Here, we report the identification of NADases on the surface of fungi such as the pathogen Aspergillus fumigatus and the saprophyte Neurospora crassa. The enzymes harbour a tuberculosis necrotizing toxin (TNT) domain and are predominately present in pathogenic species. Interestingly, N. crassa NADase (NcNADase) activity was not affected by either EGTA or Ca2+. Both AfNADase and NcNADase cleaved NAD+ and NADP+, but not their reduced counterparts, NADH and NADPH. The absence of ADP-ribosyl cyclase activity from the fungal NADase was further substantiated by its inability to convert the NAD+ analogue nicotinamide hypoxanthine dinucleotide (NHD+) to Nam and fluorescent N7-cyclic inosine diphosphoribose (N7-cIDPR), a reaction specifically observed for cyclases. These results demonstrate that fungal NADases are pure NAD glycohydrolases as they lack both cyclase and base-exchange activity.

The 1.6 Å X-ray structure of the homodimeric A. fumigatus protein reveals unique properties including N-linked glycosylation and a Ca2+-binding site whose occupancy regulates activity. The protein crystallizes in the space group P3221 with two molecules in the asymmetric unit confirming the homodimeric assembly suggested from the chromatographic analysis. The dimeric assembly is formed via an interface of 2260 Å2 of the total solvent-accessible area of 11030 Å2 (calculated with PDBePISA server), involving 66 residues, including the C-terminus which is intertwined with the other protomer. The protomers consist of two domains, an N-terminal ‘thumb’ and a C-terminal ‘palm’ domain. The thumb domain, residues 20-117, is folded containing five α-helices connected with loop regions, and the fold is stabilized by two disulfide bridges, C33-80 and C38-50. The palm domain consists of a seven-stranded central β-sheet flanked by two short α-helices and two 310 helices. The location of this binding site is at the dimerization interface, just before the C-terminus turns to intertwine with the other protomer. Noteworthy, an acetate ion, originating from the crystallization solution, is trapped in a cavity located near the domain boarder and facing the central β-sheet (strands β2, 3 and 5). The pentagonal bipyramidal coordination of the metal ion in the crystal structure, the refined density as well as the B-factors indicate that the bound metal ion is Ca2+, in line with the observed Ca2+ activation of the enzyme following EGTA treatment. The Ca2+ ion binding site is comprised of the side chains of D219, E220 and E223 as well as the main chain of S216. Each protomer is glycosylated at three asparagine residues, N45, N95 and N118 and these sites coincide with those originally predicted.

>MIFTNAILVISALLPATVLSLQHTEDSLFPARCWPDPCAGITFQNDTYVCGDPRLGPVVLPQKFPLNNELRTYARFGALCPAEFLDKWATDVAPNGTYIYPPANGFALDTEEQPILGNATLPVGMKLDRFGSEYGTFLAPLGAPYIERSLPPSNLNTFDGMYPYNYHVYQVTKEFVVGLGPIAPWFEQPGMGTQFVTYTNVLGLIDDGYLRRLDESEYDEKVEYSNPYTPGPNQDVLFQGPGHHHHHH[2x]>SMATAIATGVEHLHPLLHRN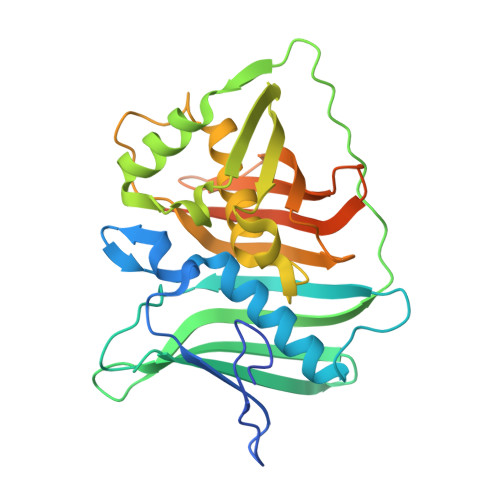VSDLRGLRYLSRFSGDESVLAEHRVNGQAVLAGAAMIVMIQAALTDALGGAVPAGRGLVISDLSWRQPFSVDAANNGELFLELSMPAAGDYRIGIYAYDQAAQLQLHCQARASTAEVQAAWLDFSSLGAQVVDVEACYQRFAAMGIEYGAGHRRLLSLVRQGDQALARIALQDPALNSGFALHPALLDAAMQGVMALLLDELEERPALLLPAGLGQCVLLADCPASLQVQIRRAPSTAPDYCFDLALFDDQGQCCAILNQLSFQPLTGASLAAGPGANIGLLCHKHWHDARPAPTA[2x]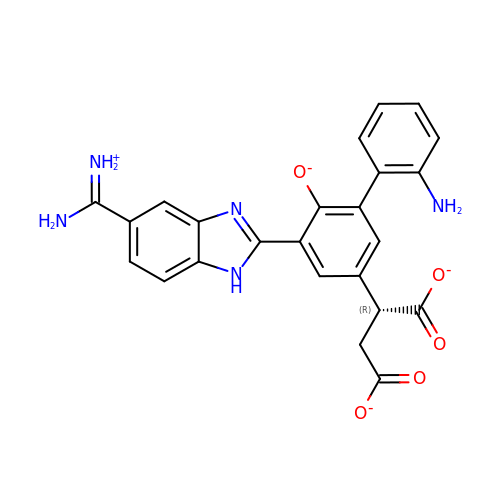2-(2'-AMINO-5-{5-[AMINO(IMINIO)METHYL]-1H-BENZIMIDAZOL-2-YL}-6-OXIDO-1,1'-BIPHENYL-3-YL)SUCCINATE | C24 H19 N5 O5 | KLIWSPNZLMZLEF-CQSZACIVSA-L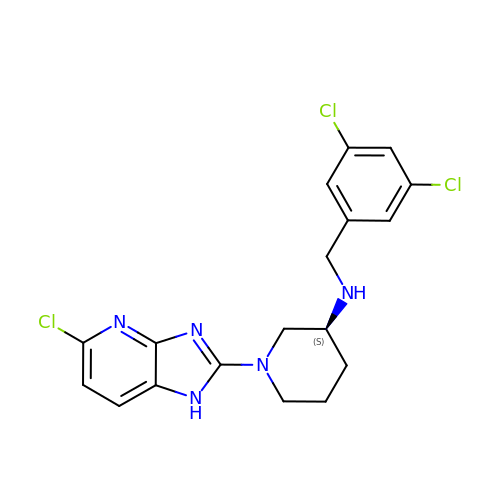(3S)-1-(5-chloro-1H-imidazo[4,5-b]pyridin-2-yl)-N-[(3,5-dichlorophenyl)methyl]piperidin-3-amine | C18 H18 Cl3 N5 | ALKJREGOUJGYEK-AWEZNQCLSA-N 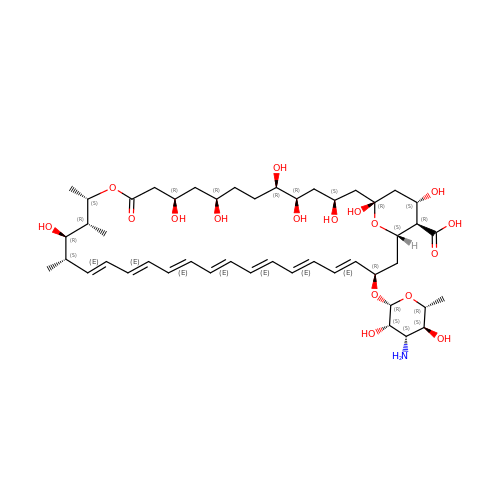Amphotericin B | C47 H73 N O17 | APKFDSVGJQXUKY-INPOYWNPSA-N>SQIRHYKWEVEYMFWAPNCNENIVMGINGQFPGPTIRANAGDSVVVELTNKLHTEGVVIHWHGILQRGTPWADGTASISQCAINPGETFFYNFTVDNPGTFFYHGHLGMQRSAGLYGSLIVDPPQGKKEPFHYDGEINLLLSDWWHQSIHKQEVGLSSKPIRWIGEPQTILLNGRGQFDCSIAAKYDSNLEPCKLKGSESCAPYIFHVSPKKTYRIRIASTTALAALNFAIGNHQLLVVEADGNYVQPFYTSDIDIYSGESYSVLITTDQ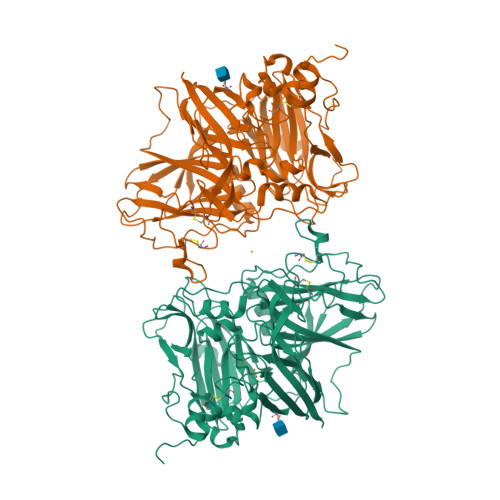NPSENYWVSVGTRARHPNTPPGLTLLNYLPNSVSKLPTSPPPQTPAWDDFDRSKNFTYRITAAMGSPKPPVKFNRRIFLLNTQNVINGYVKWAINDVSLALPPTPYLGAMKYNLLHAFDQNPPPEVFPEDYDIDTPPTNEKTRIGNGVYQFKIGEVVDVILQNANMMKENLSETHPWHLHGHDFWVLGYGDGKFSAEEESSLNLKNPPLRNTVVIFPYGWTAIRFVADNPGVWAFHCHIEPHLHMGMGVVFAEGVEKVGRIPTKALACGGTAKSLINNPKNP[2x]> MCNTYYKRVKFNLFLYTNSIEMELLAVASIIGYGLFSSQQGRETRPDRNRYAEALGSGQGLDEDYDVKPTDMVRKYRKKAEKRWKKAQVPKESGIITPNMRPSEVMPYFTSGKSMNTNTDYKQRKMELFTGGVLDGHSVSGTYKHKVEAANMFGMTPQGRVTSDGTVGNAPGDTELLKARSVNSHQYNNVLPTEQLRVGPGLGVGPEVAATGGFHQFYRQLPLNINEYKLTQLPGRLVPGGTTTGG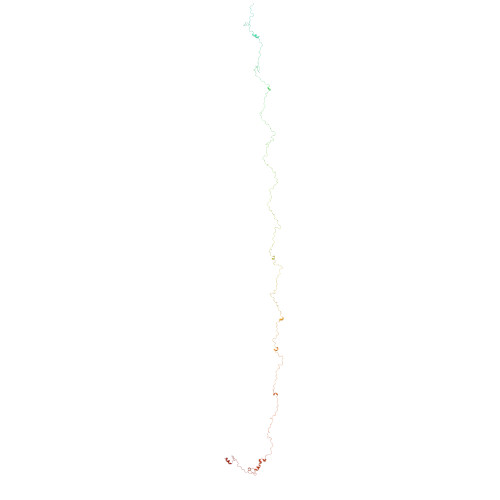KGEIQQIASVNHNPDALVLNYDDRPPEATPNGAILASTQYGKQPRGYAGLRPYEKNYEGIAEADVSALQARYLDQTRGRPRTGDGDTEPIINPNGERDGTGSYVTENMCSMTLESQRGLVNRYITPPGVTGVVQQGGEMRPEFVPETTIREQYEDIYYTGPAGTTVTPTEPMNVVELQPESRHAKRAGQDRAYTPGAGRVNNFAPAAQGAYGLKDHPTYNALQHVVSEPIEQTFLPAAQGDDDRFGTKSNVNNPWGNPASLQIANNQLAANKFNRDVTNTVNLDYDAGQPMKQQNFQPKAWIPNNTDDMKMLPLWKRKQLQAQKNKQQRK> GPLGSMNHQQQQQQQKAGEQQLSEPEDMEMEAGDTDDPPRITQNPVINGNVALSDGHNTAEEDMEDDTSWRSEATFQFTVERFSRLSESVLSPPCFVRNLPWKIMVMPRFYPDRPHQKSVGFFLQCNAESDSTSWSCHAQAVLKIINYRDDEKSFSRRISHLFFHKENDWGFSNFMAWSEVTDPEKGFIDDDKVTFEVFVQADAPHGVAWDSKKHTGYVGLKNQGATCYMNSLLQTLFFTNQLRKAVYMMPTEGDDSSKSVPLALQRVFYELQHSDKPVGTKKLTKSFGWETLDSFMQHDVQELCRVLLDNVENKMKGTCVEGTIPKLFRGKMVSYIQCKEVDYRSDRREDYYDIQLSIKGKKNIFESFVDYVAVEQLDGDNKYDAGEHGLQEAEKGVKFLTLPPVLHLQLMRFMYDPQTDQNIKINDRFEFPEQLPLDEFLQKTDPKDPANYILHAVLVHSGDNHGGHYVVYLNPKGDGKWCKFDDDVVSRCTKEEAIEHNYGGHDDDLSVRHCTNAYMLVYIRESKLSEVLQAVTDHDIPQQLVERLQEEKRIEAQKRKERQEAHLYMQVQIVAEDQFCGHQGNDMYDEEKVKYTVFKVLKNSSLAEFVQSLSQTMGFPQDQIRLWPMQARSNGTKRPAMLDNEADGNKTMIELSDNENPWTIFLETVDPELAASGATLPKFDKDHDVMLFLKMYDPKTRSLNYCGHIYTPISCKIRDLLPVMCDRAGFIQDTSLILYEEVKPNLTERIQDYDVSLDKALDELMDGDIIVFQKDDPENDNSELPTAKEYFRDLYHRVDVIFCDKTIPNDPGFVVTLSNRMNYFQVAKTVAQRLNTDPMLLQFFKSQGYRDGPGNPLRHNYEGTLRDLLQFFKPRQPKKLYYQQLKMKITDFENRRSFKCIWLNSQFREEEITLYPDKHGCVRDLLEECKKAVELGEKASGKLRLLEIVSYKIIGVHQEDELLECLSPATSRTFRIEEIPLDQVDIDKENEMLVTVAHFHKEVFGTFGIPFLLRIHQGEHFREVMKRIQSLLDIQEKEFEKFKFAIVMMGRHQYINEDEYEVNLKDFEPQPGNMSHPRPWLGLDHFNKAPKRSRYTYLEKAIKIHN;> GPPTTPKCIQCGQYLDDPDLKYGQHPPDAVDEPQMLTNEKLSIFDANESGFESYEALPQHKLTCFSVYCKHGHLCPIDTGLIEKNIELFFSGSAKPIYDDDPSLEGGVNGKNLGPINEWWITGFDGGEKALIGFSTSFAEYILMDPSPEYAPIFGLMQEKIYISKIVVEFLQSNSDSTYEDLINKIETTVPPSGLNLNRFTEDSLLRHAQFVVEQVESYDEAGDSDEQPIFLTPCMRDLIKLAGVTLGQRRAQARRQTIRHSTREKDRGPTKATTTKLVYQIFDTFFAEQIEKDDREDKENAFKRRRCGVCEVCQQPECGKCKACKDMVKFGGSGRSKQACQERRCPNMAMKEADDDEEVDDNIPEMPSPKKMHQGKKKKQNKNRISWVGEAVKTDGKKSYYKKVCIDAETLEVGDCVSVIPDDSSKPLYLARVTALWEDSSNGQMFHAHWFCAGTDTVLGATSDPLELFLVDECEDMQLSYIHSKVKVIYKAPSENWAMEGGMDPESLLEGDDGKTYFYQLWYDQDYARFESPPKTQPTEDNKFKFCVSCARLAEMRQKEIPRVLEQLEDLDSRVLYYSATKNGILYRVGDGVYLPPEAFTFNIKLSSPVK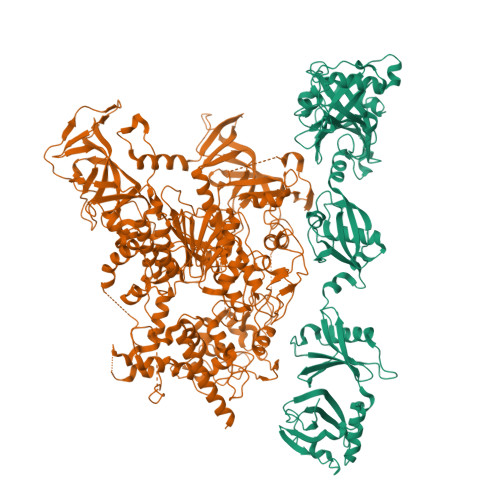RPRKEPVDEDLYPEHYRKYSDYIKGSNLDAPEPYRIGRIKEIFCPKKSNGRPNETDIKIRVNKFYRPENTHKSTPASYHADINLLYWSDEEAVVDFKAVQGRCTVEYGEDLPECVQVYSMGGPNRFYFLEAYNAKSKSFEDPPNHARSPGNKGKGKGKGKGKPKSQACEPSEPEIEIKLPKLRTLDVFSGCGGLSEGFHQAGISDTLWAIEMWDPAAQAFRLNNPGSTVFTEDCNILLKLVMAGETTNSRGQRLPQKGDVEMLCGGPPCQGFSGMNRFNSRTYSKFKNSLVVSFLSYCDYYRPRFFLLENVRNFVSFKRSMVLKLTLRCLVRMGYQCTFGVLQAGQYGVAQTRRRAIILAAAPGEKLPLFPEPLHVFAPRACQLSVVVDDKKFVSNITRLSSGPFRTITVRDTMSDLPEVRNGASALEISYNGEPQSWFQRQLRGAQYQPILRDHICKDMSALVAARMRHIPLAPGSDWRDLPNIEVRLSDGTMARKLRYTHHDRKNGRSSSGALRGVCSCVEAGKACDPAARQFNTLIPWCLPHTGNRHNHWAGLYGRLEWDGFFSTTVTNPEPMGKQGRVLHPEQHRVVSVRECARSQGFPDTYRLFGNILDKHRQVGNAVPPPLAKAIGLEIKLCMLAKARESASAKIKEEEAAKD> MGSSHHHHHHSQDPMSN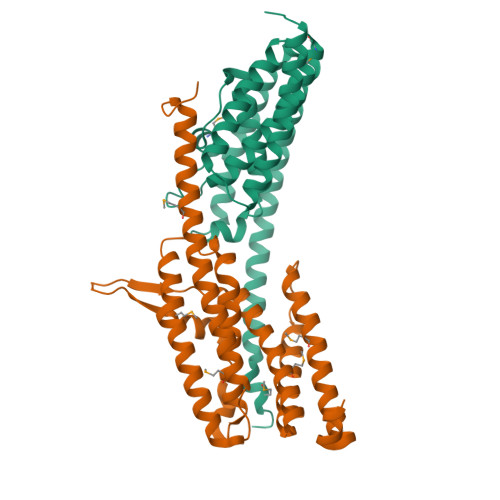FVNLDIFSNYQKYIDNEQEVRENIRIVVREIEHLSKEAQIKLQIIHSDLSQISAACGLARKQVELCAQKYQKLAELVPAGQYYRYSDHWTFITQRLIFIIALVIYLEAGFLVTRETVAEMLGLKISQSEGFHLDVEDYLLGILQLASELSRFATNSVTMGDYERPLNISHFIGDLNTGFRLLNLKNDGLRKRFDALKYDVKKIEEVVYDVSIRGLSSKEKDQQEEPAVPATE;> MPKNGGAGHRNTAPRKRQIPAAQLDEDSPIVQQFRIYSNELIMKHDRHERIVKLSRDITIESKRIIFLLHSIDSRKQNKEKVLEEARQRLNKLIAVNFRAVALELRDQDVYQFRSSYSPGLQEFIQAYTYMEYLCHEDAEGENETKSVSDWQAIQAVMQYVEESSQPKEEPTEGEDVQAIAQVESPKKFQFFVDPTEYILGLSDLTGELMRRCINSLGSGDTDTCLDTCKALQHFYSGYISLNCQRARELWRKITTMKQSVLKAENVCYNVKVRGGEAAKWGATFDQKPADEVDEGFY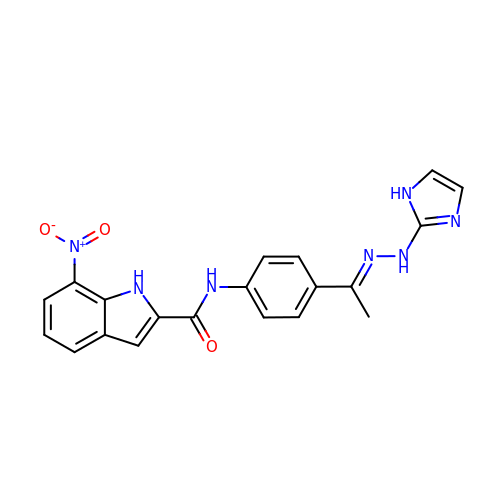N-{4-[(1E)-N-1H-IMIDAZOL-2-YLETHANEHYDRAZONOYL]PHENYL}-7-NITRO-1H-INDOLE-2-CARBOXAMIDE | C20 H17 N7 O3 | ZRMHKCSZOJQCBI-BRJLIKDPSA-N CLKs are dual-specificity kinases that are activated by autophosphorylating their own tyrosine residues and subsequently phosphorylate the serine/threonine residues of the SR protein. Later, CX-4945 was revealed to have a strong inhibitory activity on CLKs; IC50 values of 82.3 nM (CLK1), 3.8 nM (CLK2), and 90.0 nM (CLK3). In order to elucidate the selective inhibitory effect of CX-4945 on CLKs, we determined the structures of CLK1, CLK2, and CLK3 in complex with CX-4945. The overall structure of the CLK catalytic domain contained 12 β-strands and 10 α-helices that could be divided into the N-lobe and C-lobe, which are typical forms of the kinase.

In this study, for CLK1/CX-4945 complex, we used the CLK1 protein containing a single amino acid mutation (R431G) by chance. We speculate that the side chain of Arg431 might negatively affect molecular packing during crystal formation due to its flexibility. Moreover, the mutation point was far from the active site; thus, we speculated that R431G mutation was unlikely to affect the active site conformation and binding ability of CX-4945. For the β-hairpin insertion structure, CLK2 had a complete conformation, whereas CLK1 showed a partially disordered loop. In the CLK1/CX-4945 complex, the carboxy group of CX-4945 directly interacted with Lys191 located in the β4 strand and formed water-mediated interactions with Glu206 and Asp325 in the α1 helix by hydrogen bonding. The 2N of naphthyridine ring interacted with the main chain of Leu244 by hydrogen bonding. In addition the chlorine of the phenyl ring interacted with the main chain of Glu169 in the β2 strand. Val225, Leu244, Leu295, and Val324 of the C-lobe and Val167, Val175, and Phe241 of the N-lobe interacted with benzonaphthyridine by hydrophobic stacking interactions. CLK1 had the smallest and CLK3 had the largest pocket size. First, the active site of CLK1 was somewhat narrow and contained a negatively charged patch.

>[3x]MRHSKRTYCPDWDDKDWDYGKWRSSSSHKRRKRSHSSAQENKRCKYNHSKMCDSHYLESRSINEKDYHSRRYIDEYRNDYTQGCEPGHRQRDHESRYQNHSSKSSGRSGRSSYKSKHRIHHSTSHRRSHGKSHRRKRTRSVEDDEEGHLICQSGDVLSARYEIVDTLGEGAFGKVVECIDHKAGGRHVAVKIVKNVDRYCEAARSEIQVLEHLNTTDPNSTFRCVQMLEWFEHHGHICIVFELLGLSTYDFIKENGFLPFRLDHIRKMAYQICKSVNFLHSNKLTHTDLKPENILFVQSDYTEAYNPKIKRDERTLINPDIKVVDFGSATYDDEHHSTLVSTRHYRAPEVILALGWSQPCDVWSIGCILIEYYLGFTVFPTHDSKEHLAMMERILGPLPKHMIQKTRKRKYFHHDRLDWDEHSSAGRYVSRACKPLKEFMLSQDVEHERLFDLIQKMLEYDPAKRITLREALKHPFFDLLKKSI> MASTNTNLQKAIDLASKAAQEDKAGNYEEALQLYQHAVQYFLHVVKYEAQGDKAKQSIRAKCTEYLDRAEKLKEYLKKKEKKPQK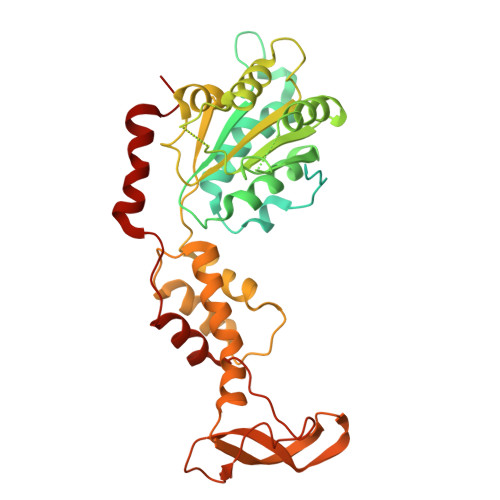PVKEEQSGPVDEKGNDSDGEAESDDPEKKKLQNQLQGAIVIERPNVKWSDVAGLEGAKEALKEAVILPIKFPHLFTGKRTPWRGILLFGPPGTGKSYLAKAVATEANNSTFFSISSSDLVSKWLGESEKLVKNLFQLARENKPSIIFIDEIDSLCGSRSENESEAARRIKTEFLVQMQGVGVDNDGILVLGATNIPWVLDSAIRRRFEKRIYIPLPEAHARAAMFRLHLGSTQNSLTEADFQELGRKTDGYSGADISIIVRDALMQPVRKVQSATHFKKVRGPSRADPNCIVNDLLTPCSPGDPGAIEMTWMDVPGDKLLEPVVSMWDMLRSLSSTKPTVNEQDLLKLKKFTEDFGQEG> GHPMSPGVFFDSDKGKTHSSGKVLYNARIIPYRGSWLDFE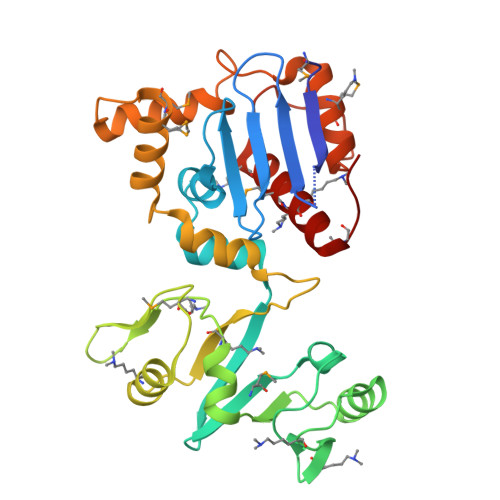FDPKDNLFVRIDRRRKLPATIILRALNYTTEQILDLFFEKVIFEIRDNKLQMELVPERLRGETASFDIEANGKVYVEKGRRITARHIRQLEKDDVKLIEVPVEYIAGKVVAKDYIDESTGELICAANMELSLDLLAKLSQSGHKRIETLFTNDLDHGPYISETLRVDPTNDRLSALVEIYRMMRPGEPPTREAAESLFENLFFSEDRYDLSAVGRMKFNRSLLREEIEGSGILSKDDIIDVMKKLIDIRNGKGEVD>[2x]MQTKERYQLQRLTLLALLTAMCVVLRIFKIIDIPNVQPVTDIIMLTTLELGAGTGILLAILVMVISNIFLGFGIWTLPQIFAYAACALTVALFARLLPLKSRKFFWLQELLAGFLGLEYGFFVSLGMAGWGGWAAFIAYWVSGLTFDLYHAAGNLAFYPIFYLPLVLGLDRFKKKAGWKQNA;>[2x]MHHHHHHHHHHGENLYFQGSDNIISFDHVTFTYPDSPRPALSDLSFAIERGSWTALIGHNGSGKSTVSKLINGLLAPDDLDKSSITVDGVKLGADTVWEVREKVGIVFQNPDNQFVGATVSDDVAFGLENRAVPRPEMLKIVAQAVADVGMADYADSEPSNLSGGQKQRVAIAGILAVKPQVIILDESTSMLDPEGKEQILDLVRKIKEDNNLTVISITHDLEEAAGADQVLVLDDGQLLDQGKPEEIFPKVEMLKRIGLDIPFVYRLKQLLKERGIVLPDEIDDDEKLVQSLWQLNSKM;>[2x]MAIKFENVSYVYSPGSPLEAIGLDQLNFSLEEGKFIALVGHTGSGKSTLMQHFNALLKPTSGKIEIAGYTITPETGNKGLKDLRRKVSLAFQFSEAQLFENTVLKDVEYGPRNFGFSEDEAREAALKWLKKVGLKDDLIEHSPFDLSGGQMRRVALAGVLAYEPEII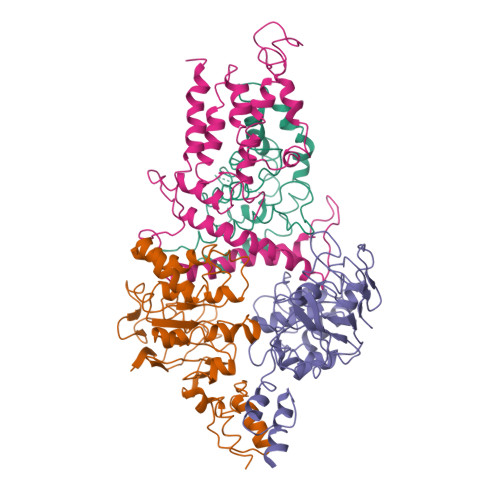CLDEPAAGLDPMGRLEMMQLFKDYQAAGHTVILVTHNMDDVADYADDVLALEHGRLIKHASPKEVFKDSEWLQKHHLAEPRSARFAAKLEAAGLKLPGQPLTMPELADAIKQSLKGGEHE;>[2x]MSKIIIGRYLPGTTFVYRVDPRAKLLTTFYFIIMIFLANNWVSYLVISIFGLAYVFATGLKARVFWDGVKPMIWMIVFTSLLQTFFMAGGKVYWHWWIFTLSSEGLINGLYVFIRFAMIILVSTVMTVTTKPLEIADAMEWMLTPLKLFKVNVGMISLVISIALRFVPTLFDQTVKIMNAQRSRGADFNDGGLVKRAKSVVPMLVPLFIDSLEVALDLSTAMESRGYKGSEGRTRYRILEWSKVDLIPVAYCLLLTILMITTRKH>[2x]SVVLPVAKRGEDILKLIAAPVSA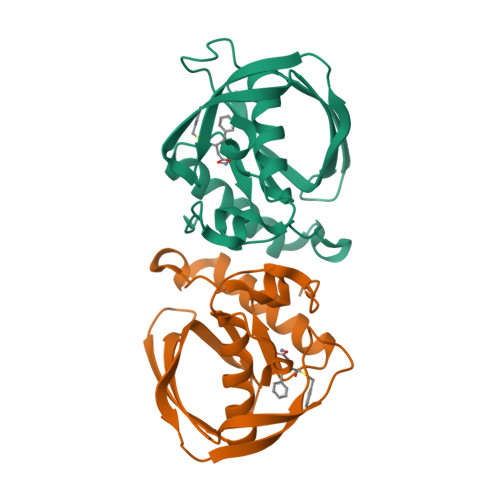NELNSNWLYQLADAMHATMLERNGVGIAAPQVYISKRVIIVASRPNPRYPDAPEMNAVVMVNPEILEFSSETCLGEEGCLSVPDERGQVERAEMVKVKYLTLQGEAVETIFHGFPARIVQHEVDHLNGILFVERIS> MKARTG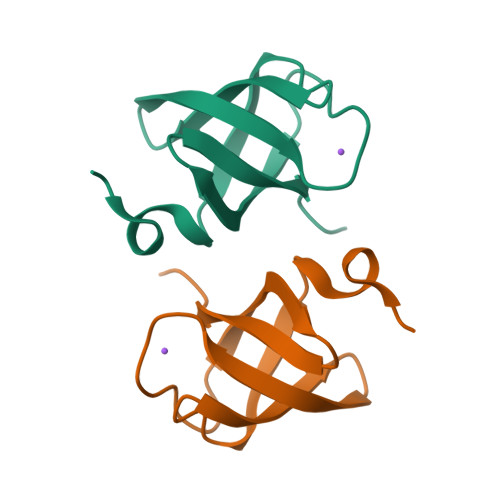KEEMIGLIGTVVEELNPEGMIKVRGELWKARSKFNGKIEKGEKVRVVDMDGLTLIVVRERKEGGEKLEHHHHHH>KFGWIKGV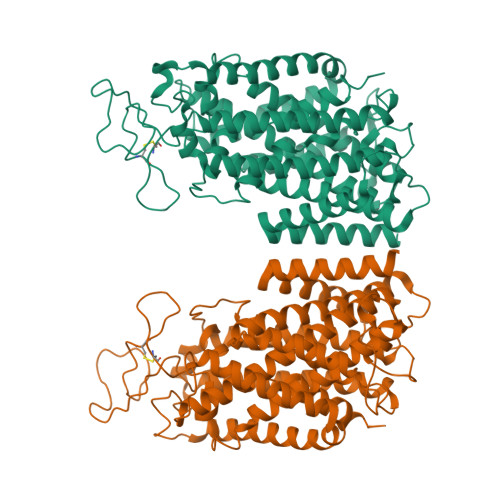LVRCMLNIWGVMLFIRMTWIVGQAGIAYSCIIVIMATVVTTITGCSTSAIATNGFVRGGGAYYLISRSLGPEFGGSIGLIFAFANAVAVAMYVVGFAETVVELLMDSGLLMIDQTNDIRVIGTITVILLLGISVAGMEWEAKAQIFLLVILITAIFNYFIGSFIAVDSKKKFGFFSYDAGILAENFGPDFRGQTFFSVFSIFFPAATGILAGANISGDLADPQMAIPKGTLLAILITGLVYVGVAISAGACIVRDATGIESNFTLISNCTDAACKYGYDFSSCRPTVEGEVSSCKFGLHNDFQVMSVVSGFSPLISAGIFSATLSSALASLVSAPKVFQALCKDNIYPGIAIFGKGYGKNNEPLRGYFLTFGIALAFILIAELNVIAPIISNFFLASYALINFSVFHASLANSPGWRPSFKYYNMWASLAGAILCCVVMFIINWWAALLTNVIVLSLYIYVSYK[2x]> GSSDDEDSVRYLLYMAELRYEQGNPEKAKKILEMAEFIAKRNNNEELERLVREVKKRL

The structure is that of a small (58 residues) engineered protein, LCB2, which was developed in Baker’s laboratory as a blocking ligand of the SARS-CoV-2 spike protein. It was envisioned that solutions of mini-proteins such as LCB2 could be used in the form of a nasal spray to confer temporary protection against the coronavirus infection. While LCB2 was validated by means of biolayer interferometry experiments and tested in cell culture assays employing live virus, it has not been developed further.

We found that AlphaFold3, AlphaFold2, MultiFOLD, Rosetta, RoseTTAFold and trRosetta all produced successful MR models for this three-helix bundle 58-residue protein, while some of the older predictors failed. While the initial models showed appreciable variability (up to 0.87 Å) and differed substantially from the final coordinates (up to 1.08 Å), the structure determination process fully converged, resulting in six refined models within 0.25 Å from each other. All structures include residues from 4 to 58, with no alternative conformations; they also include from 1 to 4 glycerol molecules and between 18 and 24 water molecules. The situation with the loop 42–44 led us to suggest that its conformation in the crystallographic structure is influenced by a crystal contact. Indeed, it turns out that residue Asn43 at the center of the loop forms an intermolecular side-chain-to-backbone hydrogen bond with the amide group of residue Glu46 in the symmetry-related protein molecule. This hydrogen bond apparently leads to stretching out of the loop, thus causing the difference between the computer-generated model and the actual structure, see Fig. 1(g). Comparing the six structural solutions, we observe that a number of surface side chains have been solved with different conformations. Interestingly, for each individual structure the electron density is consistent with a single rotameric state and offers no direct evidence of conformational heterogeneity. We thus conclude that the six LCB2 structures obtained in this study can be grouped into a multiconformer ensemble, where structural variations are representative of protein’s conformational dynamics. While Rwork/Rfree of the individual structures is at best 0.208/0.240, the six-member ensemble yields significantly improved values, 0.187/0.220.>[12x]QLGAIENGLESGSANACPDAILIFARGSTEPGNMGI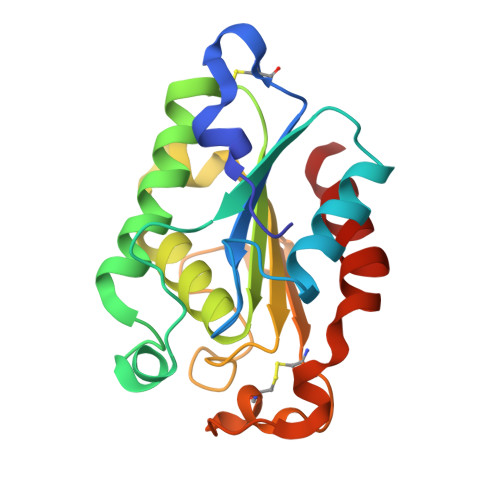TVGPALANGLESHIRNIWIQGVGGPYDAALATNFLPRGTSQANIDEGKRLFALANQKCPNTPVVAGGYSQGAALIAAAVSELSGAVKEQVKGVALFGYTQNLQNRGGIPNYPRERTKVFCNVGDAVCTGTLIITPAHLSYTIEARGEAARFLRDRIRA> MGHHHHHHGEGDVESIEKFLSTFKILPPLRDYKEFGPIQEIVRSPNMGNLRGKLIATLMENEPNSITSSAVSPGETPYLITGSD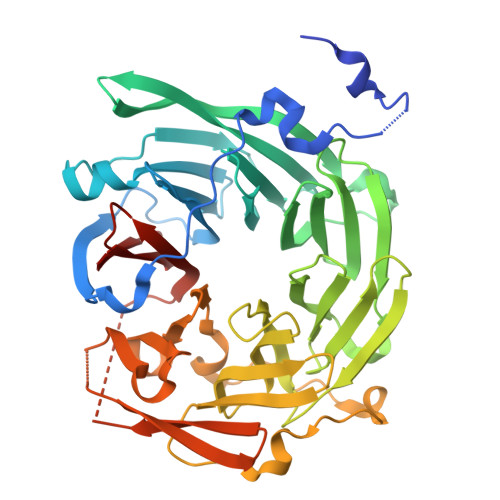QGVIKIWNLKEIIVGEVYSSSLTYDCSSTVTQITMIPNFDAFAVSSKDGQIIVLKVNHYQQESEVKFLNCECIRKINLKNFGKNEYAVRMRAFVNEEKSLLVALTNLSRVIIFDIRTLERLQIIENSPRHGAVSSICIDEECCVLILGTTRGIIDIWDIRFNVLIRSWSFGDHAPITHVEVCQFYGKNSVIVVGGSSKTFLTIWNFVKGHCQYAFINSDEQPSMEHFLPIEKGLEELNFCGIRSLNALSTISVSNDKILLTDEATSSIVMFSLNELSSSKAVISPSRFSDVFIPTQVTANLTMLLRKMKRTSTHSVDDSLYHHDIINSISTCEVDETPLLVACDNSGLIGIFQ>AEIRKLKNYINGEWVESKTDQYEDVVNPATKEVLCQVPISTKEDIDYAAQTAAEAFKTWSKVAVPRRARILFNFQQLLSQHKEELAHLITIENGKNTKEALGEVGRGIENVEFAAGAPSLMMGDSLASIATDVEAANYRYPIGVVGGIAPFNFPMMVPCWMFPMAIALGNTFILKPSERTPLLTEKLVELFEKAGLPKGVFNVVYGAHDVVNGILEHPEIKAISFVGSKPVGEYVYKKGSENLKRVQSLTGAKNHTIVLNDANLEDTVTNIVGAAFGSAGERCMACAVVTVEEGIADEFMAKLQEKVADIKIGNGLD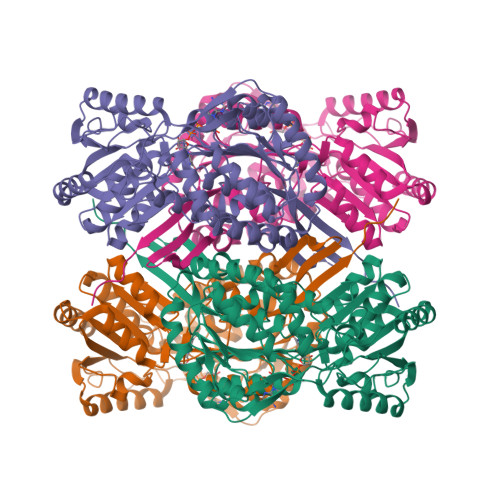DGVFLGPVIREDNKKRTLSYIEKGLEEGARLVCDGRENVSDDGYFVGPTIFDNVTTEMTIWKDEIFAPVLSVIRVKNLKEAIEIANKSEFANGACLFTSNSNAIRYFRENIDAGMLGINLGVPAPMAFFPFSGWKSSFFGTLHANGKDSVDFYTRKKVVTARYPAPDFN[4x]> STENLYFQSNADSVQNHTFEVENNTINGLELVEEQVHILYAMVLQTHADVQLLKEQQ;> TQWDDWVDKMENLNHDILTT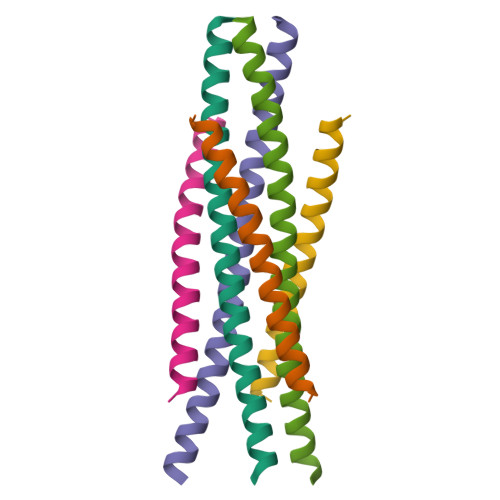LHTARNNLEQSMITFNT> MNNTFKFLHQVISKLTLKAQVPNYGQYSHSLKRPINPKVVVFGNSSRAYELISSQFRNFNHVNGLELKGQEDNIQAN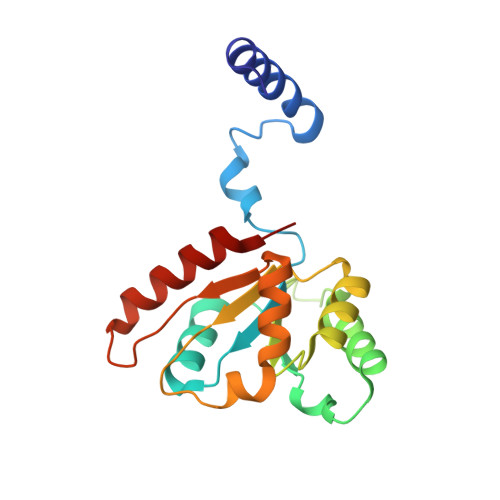KVAQSVLSINDGFQDGYYITDFPQNSKQAERLDLITDGVNLALYIKDPSDKVTVTRQQEAIDYYRKTGALVEFEVDPRGDLEEQVKQLSNQVLNGYKH>MPKLVTWMNNQRVGELTKLANGAHTFKYAPEWLASRYARPLSLSLPLQRGNITSDAVFNFFDNLLPDSPIVRDRIVKRYHAKSRQPFDLLSEIGRDSVGAVTLIPEDETVTHPIMAWEKLTEARLEEVLTAYKADIPLGMIREENDFRISVAGAQEKTALLRIGNDWCIPKGITPTTHIIKLPIGEIRQPNATLDLSQSVDNEYYCLLLAKELGLNVPDAEIIKAGNVRALAVERFDRRWNARRTVLLRLPQEDMCQTFGLPSSVKYESDGGPGIARIMAFLMGSSEALKDRYDFMKFQVFQWLIGATQGHAKNFSVFIQAGGSYRLTPFYDIISAFPVLGGTGIHISDLKLAMGLNASKGKKTAIDKIYPRHFLATAKVLRFP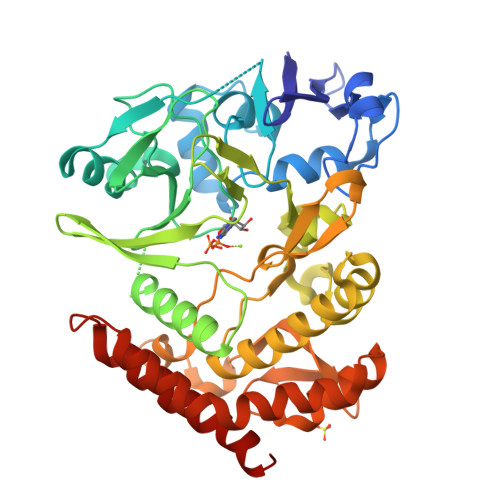EVQMHEILSDFARMIPAALDNVKTSLPTDFPENVVTAVESNVLRLHGRLSREYGSK[2x]>MSTSSHTVLLIQTSPRLDSRTWGDYESVTDALDALCKMFEDFLSKKSAAPVTYDVSQVYEFLDKLSDVSMMIFNRETGQYIGRTRAWIKQQVYEMMRGRCQHPGSSGSSGSSGSSG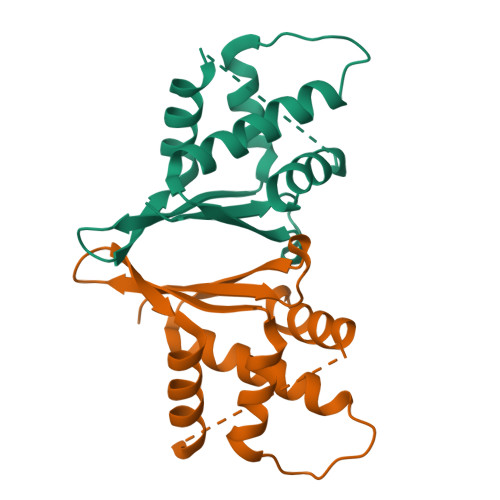SSGSSGSSEDIKDSVFKVLHAEEEPRGAD[2x]> SMEEPEEPADSGQSLVPVYIYSPEYVSMCDSLAKIPKRA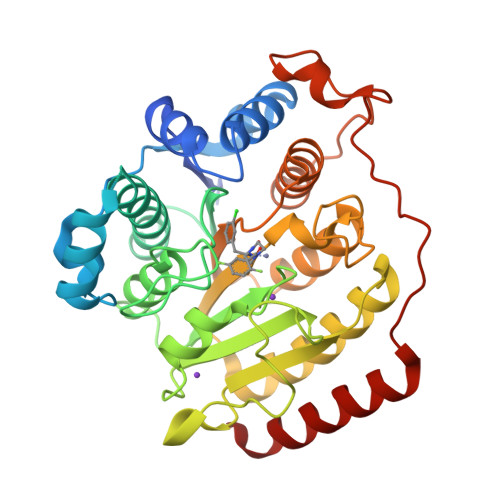SMVHSLIEAYALHKQMRIVKPKVASMEEMATFHTDAYLQHLQKVSQEGDDDHPDSIEYGLGYDCPATEGIFDYAAAIGGATITAAQCLIDGMCKVAINWSGGWHHAKKDEASGFCYLNDAVLGILRLRRKFERILYVDLDLHHGDGVEDAFSFTSKVMTVSLHKFSPGFFPGTGDVSDVGLGKGRYYSVNVPIQDGIQDEKYYQICESVLKEVYQAFNPKAVVLQLGADTIAGDPMCSFNMTPVGIGKCLKYILQWQLATLILGGGGYNLANTARCWTYLTGVILGKTLSSEIPDHEFFTAYGPDYVLEITPSCRPDRNEPHRIQQILNYIKGNLKHVV>[4x]MGSDKIHHHHHHMKIDILDKGFVELV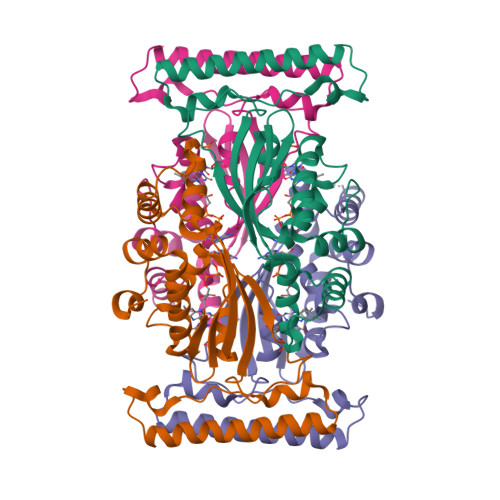DVMGNDLSAVRAARVSFDMGLKDEERDRHLIEYLMKHGHETPFEHIVFTFHVKAPIFVARQWFRHRIASYNELSGRYSKLSYEFYIPSPERLEGYKTTIPPERVTEKISEIVDKAYRTYLELIESGVPREVARIVLPLNLYTRAFATVNARSLMNFLNLRADSHAQWEIQQYALAIARIFKEKCPWTFEAFLKYAYKGDILKEVQV>MACTGPSLPSAFDILGAAGQDKLLYLKHKLKTPRPGCQGQDLLHAMVLLKLGQETEARISLEALKADAVARLVARQWAGVDSTEDPEEPPDVSWAVARLYHLLAEEKLCPASLRDVAYQEAVRTLSSRDDHRLGELQDEARNRCGWDIAGDPGSIRTLQSNLGCLPPSSALPSGTRSLPRPIDGVSDWSQGCSLRSTGSPASLASNLEISQSPTMPFLSLHRSPHGPSKLCDDPQASLVPEPVPGGCQEPEEMSWPPSGEIASPPELPSSPPPGLPEVAPDATSTGLPDTPAAPETSTNYPVECTEGSAGPQSLPLPILEPVKNPCSVKDQTPLQLSVEDTTSPNTKPCPPTPTTPETSPPPPPPPPSSTPCSAHLTPSSLFPSSLESSSEQKFYNFVILHARADEHIALRVREKLEALGVPDGATFCEDFQVPGRGELSCLQDAIDHSAFIILLLTSNFDCRLSLHQVNQAMMSNLTRQGSPDCVIPFLPLESSPAQLSSDTASLLSGLVRLDEHSQIFARKVA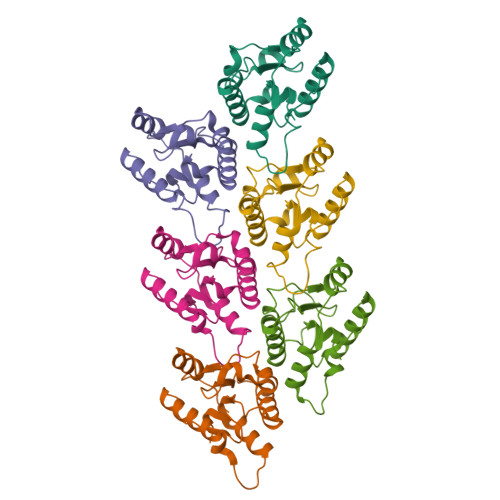NTFKPHRLQARKAMWRKEQD[6x]Type III secretion systems (T3SS) are bacterial macromolecular machines that facilitate transport of protein substrates across the bacterial cell envelope. Most building blocks of the virulence associated T3SS or injectisome have a homologue in flagella and one of the most highly conserved parts of the system is a set of transmembrane proteins known collectively as the export apparatus (EA). The FlhA/SctV cytoplasmic domain is known to form a nonameric ring underneath FliPQR-FlhB/SctRSTU, but the full-length FlhA/SctV complex remains poorly characterised. Open and closed states have been described, with the open state being competent for chaperone-substrate complex binding, while the closed state has been proposed to be responsible for binding early substrates.

Out of the identified proteins we chose FlhA from the lateral flagella of Vibrio parahaemolyticus (Vp-FlhA) and SctV from Yersinia enterocolitica (Ye-SctV) for further studies, as both could be produced in large quantities at high purity using the gentle detergent LMNG. In contrast, Vp-FlhA was found to form the predicted nonameric complex and we imposed C9 symmetry for particle refinement, resulting in a 3.8 Å volume of the cytoplasmic domain but little detail in the transmembrane domain. A striking feature of both structures is the N-terminal density of the cytoplasmic domain, formed by FlhAL/SctVL, which reaches out to bind to the adjacent protomer, demonstrating this well studied interaction for the first time in the context of the full-length protein in both flagellar and injectisome T3SS. In both of our structures a hydrophobic residue, Trp350 in Vp-FlhA and Phe367 in Ye-SctV, sticks into a hydrophobic groove on the neighbouring subunit. This residue in FlhA has previously been shown to be involved in ring formation of the cytoplasmic domain of FlhA. Comparison of our structures with FlhA from S. Typhimurium, St-FlhA, in the open state and Sf-SctV, which is in the closed state shows that both of our complexes are in the open state, with Ye-SctV being the first example of an SctV homologue in the open state. We simulated the movement of FlhAL by overlaying one subunit of Vp-FlhA onto the SD3 or SD2 subdomain of the closed Sf-SctV structure. This demonstrates that adoption of the closed state in one subunit would affect the neighbouring subunit, potentially propagating the conformational change in a wave around the ring. Our structures are not affected by crystallisation artefacts and are in the context of the full-length protein, suggesting that the open state is the default state in the absence of other factors. Our structures also suggest that at least in the open state the residues known as FlhAL/SctVL, which have previously been described as the linker between cytoplasmic and membrane domains, do not form part of this linker but are part of the cytoplasmic domain.

>MLTRLKQLQTSTKGYIGIPIVLLMILAMVILPLPPLLLDALFTFNIVLAILVLLVSTTAKRPLDFSVFPTILLVATLLRLTLNVASTRIVLLEGHNGGDAAGKVIQAFGEVVIGGNYVVGMVVFIILMIINFVVITKGGERISEVSARFTLDALPGKQMAIDADLNAGLIDQETARLRRKEVANEADFHGSMDGASKFVRGDAVAGLLILFINIIGGISIGVFEHGLPASEAFKTYALLTIGDGLVAQIPSLLLATAAAIIVTRINDSDNGMSETMQKQLLATPATLFTVAGIMAVIGMVPGMPHLAFFAFAGALGFAGWRQSKKPVQDTQIEQVEALSQAMQEEDTPLTWDDIPHVHTLSLALGYRLVHLVNKDQGAPLSQRIRGVRRNLSEQVGFLLPEVRIRDNLSLKPNQYTISLNGEVIEQGFIEPERLMAIAVGDTYGEIDGILGSDPAYQLPAVWIEHQDKAKALNMGYQVVDDGTVIATHISKIMKTNLAELFTHDDVEAMTQRLTQQAPKLAEALAAALNPAQQLKVYRQLLLDQVPLKDIRTIANTMLESSENTKDPILLAADVRCALKRTLVNLIAGQKPELNVYALSDELEQMLLTSLQQAQASGTVVLDSFPIEPNILGQFQQNLPLIRQQLKQQGLPPILLVMPQLRPLLARYARTFTQGLAVLSYNEIPENKQINVVGNLGENLYFQ[9x]Calcineurin (CN) is a Ca2+/calmodulin (CaM)-dependent, serine, threonine-specific protein phosphatase that controls T-cell activation and is critical for numerous cellular functions. The CN complex is composed of a catalytic (CnA) and regulatory (CnB) subunit that binds Ca2+, and is activated by Ca2+–CaM2. Here we report the crystal structures of fungal CN ternary complexes with FKBP12-FK506 from highly clinically relevant human fungal pathogens: A. fumigatus, C. albicans, C. neoformans, and Coccidioides immitis, reflecting the common invasive fungal pathogens, including a mold, yeasts, and a dimorphic endemic fungus. Each complex has three components: (1) the CnA subunit with catalytic domain and the BBH, (2) the CnB subunit, with four EF hands bound to Ca2+ and wrapping around the BBH, and (3) FKBP12 bound to FK506, interfacing with CnA/CnB.

Crystal structures of CN–FK506-FKBP12 ternary complexes from four fungi were determined by molecular replacement to resolutions between 1.85 and 3.30 Å. Despite sequence variations between the mammalian and fungal counterparts of CN and FKBP12, the X-ray characterized ternary complexes reveal high structural homology. A flexible hinge in CnA separates the catalytic domain from the BBH, which forms the composite surface for FKBP12-FK506-complex binding. Fungal CnB structures are also conserved, with two well-resolved C-terminal EF-hands close to the FKBP12-FK506 binding surface and the two distal N-terminal EF-hands showing varying degrees of disorder, suggesting interaction with FKBP12-FK506 may stabilize the C-terminal EF-hands. The interface between CN and FKBP12-FK506 complexes is conserved across fungi, but differences are notable in the binding surfaces of FKBP12 and CnA in fungi versus mammalian proteins. While the CnA and CnB interacting residues within 5–8 Å of FK506 in human and fungi are conserved, fungal FKBP12s differed in 4 of the 17 interacting residues, as well as other residues surrounding the 40s and 80s loops.

>[2x]MGSSHHHHHHSSGLVPRGSTDDGEKYSTVERAVKSVDPPATFKPKDEQVFYPNGKPNHQFLKQHFIHEGRLHEHQAIQILKQATHLLSKEPNLLSVPAPVTICGDVHGQYYDLMKLFEVGGDPASTKYLFLGDYVDRGSFSIECLLYLYSLKINYPDTFWMLRGNHECRHLTEYFTFKNECLHKYSEELYEECLVSFNALPLAAIMNEQFFCVHGGLSPQLTSLDSLRKLHRFREPPTKGLMCDLLWADPIEEYDDDNLDQEYVTNVVRGCSFAFTYKAACKFLDRTKLLSVIRAHEAQNAGYRMYKRTKTMGFPSLLTMFSAPNYLDSYNNKAAVLKYENNVMNIRQFNASPHPYWLPHFMDVFTWSLPFVGEKVTDMLVSILNVCTEEELDEDLPFSEAEIGVTPTTTT;>[2x]MGANASILDGFIEDTNFSIEEIDRLRKRFMKLDKDGSGQIDKQEFLSIPGISSNPLATRLMDVFDKDGDGSIDFEEFITGLSAFSGKSDNLNKLRFAFNIYDIDRDGYIGNGELFIVMKMMVGKNLKDEELQQIVDKTLMEADLDGDGKLNFEEFKNAVNTDTIANTLTLNMF;>[2x]GSHMSEELPQIEIVQEGDNTTFAKPGDTVTIHYDGKLTNGKEFDSSRKRGKPFTCTVGVGQVIKGWDISLTNNYGKGGANLPKISKGTKAILTIPPNLAYGPRGIPPIIGPNETLVFEVELLGVNGQ>GVSTAVAQDFTIAAKHAIAVEANTGKILYEKDATQPVEIASITKLITVYLVYEALENGSITLSTPVDISDYPYQLTTNSEASNIPMEARNYTVEELLEATLVSSANSAAIALAEKIAGSEKDFVDMMRAKLLEWGIQDATVVNTTGLNNETLGDNIYPGSKKDEENKLSAYDVAIVARNLIKKYPQVLEITKKPSSTFAGMTITSTNYMLEGMPAYRGGFDGLKTGTTDKAGESFVGTTVEKGMRVITVVLNADHQDNNPYARFTAT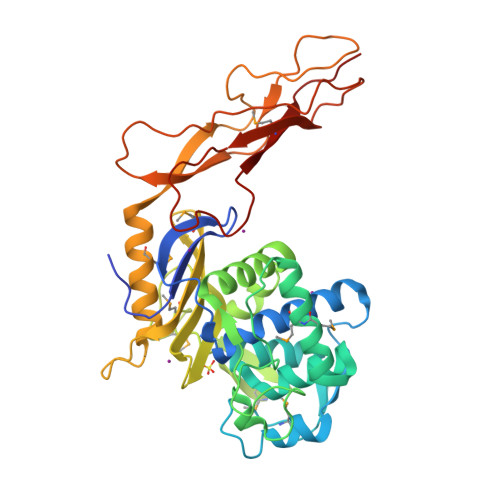SSLMDYISSTFTLRKIVQQGDAYQDSKAPVQDGKEDTVIAVAPEDIYLIERVGNQSSQSVQFTPDSKAIPAPLEAGTVVGHLTYEDKDLIGQGYITTERPSFEMVADKKIEK[4x]> MADNEKLDNQRLKNFKNKGRDLETMRRQRNEVVVELRKNKRDEHLLKRRNVPHEDICEDSDIDGDYRVQNTSLEAIVQNASSDNQGIQLSAVQAARKLLSSDRNPPIDDLIKSGILPILVHCLERDDNPSLQFEAAWALTNIASGTSEQTQAVVQSNAVPLFLRLLHSPHQNVCEQAVWALGNIIGDGPQCRDYVISLGVVKPLLSFISPSIPITFLRNVTWVMVNLCRHKDPPPPMETIQEILPALCVLIHHTDVNILVDTVWALSYLTDAGNEQIQMVIDSGIVPHLVPLLSHQEVKVQTAALRAVGNIVTGTDEQTQVVLNCDALSHFPALLTHPKEKINKEAVWFL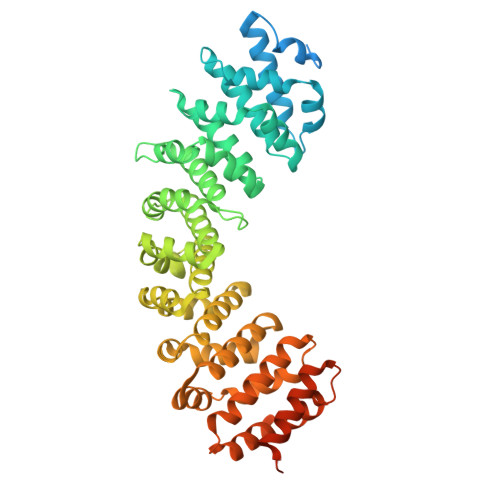SNITAGNQQQVQAVIDANLVPMIIHLLDKGDFGTQKEAAWAISNLTISGRKDQVAYLIQQNVIPPFCNLLTVKDAQVVQVVLDGLSNILKMAEDEAETIGNLIEECGGLEKIEQLQNHENEDIYKLAYEIIDQFFSSDDIDEDPSLVPEAIQGGTFGFNSSANVPTEGFQF> MLRRSLLAFPWWNFQTEHRQRCVLMYGGARTKNTHNANHRVFIKKYKRNAFPNRTRHHWAVSMTGVLSQRPRRMPWPYDLTSLIFNQPRQGSDKIGYVVGTSMLKTAVVATNHMVYYPKFNQRVSRTKRFFAHDEDLACVEGDLVHIKQCRK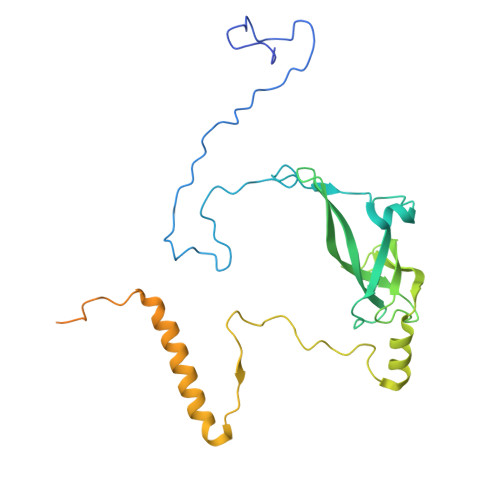ISKYKHYYVFSILEPNVEGRERLKLGLKAVPPPLFGYPVSRRIVKLNLTSTEGTQEKLAAAIQEHVQDAYRFSGPTPDQPRNRLADPVTFEDANNMIAPNAPAAAALDASDSPPLLDRGEYTEVEQDTRNKKGDDYWMNLQPKEKYDFKSFKKSP In Streptomyces scabiei, the main causative agent of common scab disease of root and tuber crops, the interaction between the substrate-binding protein (SBP) CebE (CebEscab) and cellotriose released by the plant host (K D in the nanomolar range) is the first event for the onset of its pathogenic lifestyle. CebE is the sugar-binding component of the ABC transporter, proteins CebF and CebG form the transporter permease, and the energy for active cello-oligosaccharide transport is provided by the multiple sugar importer ATPase MsiK. CebEscab adopts a cluster B-type substrate-binding protein (SBP)-fold as described by Berntsson et al.. It is composed of two domains connected by three hinge regions.

We obtained the crystallographic structure of CebEscab in complex with cellotriose at a 1.55-Å resolution. The CebEscab structure contains residues 62–454. The elongated ligand binding pocket is located at the interface between the two domains. An electron density corresponding to the whole cellotriose molecule is observed in the ligand binding pocket, clearly establishing the two β-1,4 links between the three β-D-glucoses. The reducing end (D-Glc1) is more inserted in Domain 2, whereas the non-reducing end (D-Glc3) makes more interactions with Domain 1. Cellotriose is stabilized in the pocket by a few hydrophobic interactions and numerous H-bonds, nine of them being mediated by eight water molecules surrounding the ligand. D-Glc3 provides the highest contribution to the binding of cellotriose, being involved in ten H-bonds and three hydrophobic interactions with the sidechain of W303 (parallel stacking), F70, and M123. D-Glc1 and D-Glc2 follow with 7 and 6 H-bonds, respectively, the latter being involved in an additional hydrophobic interaction with F282. It, therefore, seems that an important part of the interactions between Domains 1 and 2 is mediated by the cellotriose molecule itself. The ligand would, therefore, be responsible for the closing of the sugar-binding pocket, a phenomenon termed as induced-fit ligand binding mechanism.

> HHHHHHSSGLVPRGSHDDGKDEEGGSSDGGGGGKTKITLGLFGTAGFEESGLYKEYEKLHPDVDIQQTVVERNENYYPALLNHLTTGSGLQDIQMVEVGNIAEIVGTQSDKLLDLSKYGKESDYLPWKWSQGSTSGGQTVALGTDVGPMAICYRKDLFEAAGLPSDREEVGKLWTGSWDKFVDAGNQYKKKAPKGTTFLDSPGGLLQAILSSEKDRFYDASGKVIYKTNPAVKSAFDLTAKAAKAGLVGNQTQFQPAWDTTIANSKFAAMSCPPWMLGYIKGKSKPEAAGKWDIAQAPKSGNWGGSFLSVPKNGKNAEEAAKLAAWLTAPEQQAKLFAVQGSFPSTPAAYDSAAVKDAKNDMTGDAPIGTIFAEAAKNIPVQTIGPKDQIIQQGLTDNGVILVTQGKSASDAWKNAVKTIDNALDK>[2x]MDSEEVNERVKQLAEKAKEATDKEEVIEIVKELAELAKQSTDPNLVAEVVRALTEVAKTSTDTELIREIIKVLLELASKLRDPQAVLEALQAVAELARELAEKTGDPIAKECAEAVSAAAE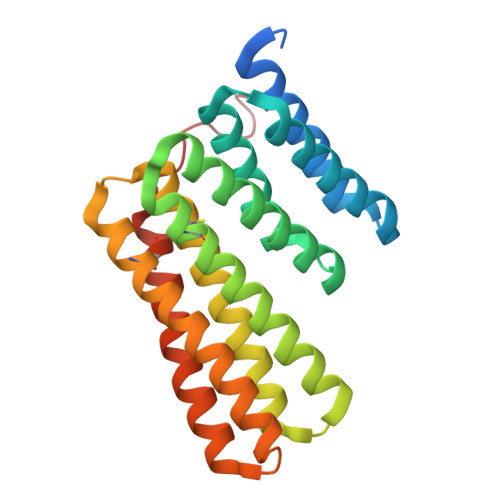AVKKAADLLKRHPGSEAAQAALELAKAAAEAVLIACLLALDYPKSDIAKKCIKAASEAAEEASKAAEEAQRHPDSQKARDEIKEASQKAEEVKERCERAQEHPNAGWLEHHHHHH> MLTEGISIQSYDGHTFGALVGSPAKAPAPVIVIAHEILGVNAFMRETVSWLVDQGYAAVCPDLYARQ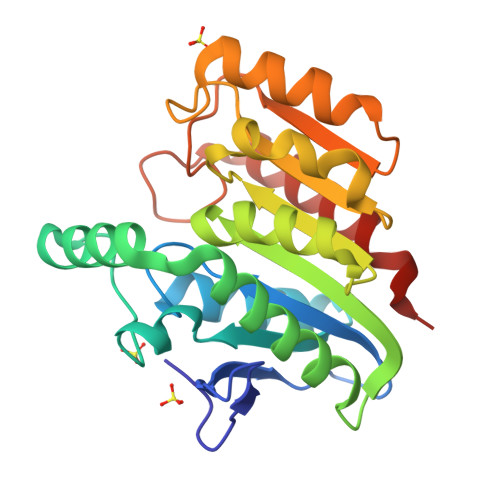APGTALDPQDEAQREQAYKLWQAFDMEAGVGDLEAAIRYARHLPYSNGKVGLVGYSLGGALAFLVAAKGCVDRAVGYCGVGLEKQLDKVPEVKHPALFHMGGQDHFVPAPSRQLITEGFGANPLLQVHWYEGAGHSFARTGSSDYVASAAALANERTLDFLAPLQSNKP(2E,4E)-2-HYDROXY-6-OXO-6-PHENYLHEXA-2,4-DIENOIC 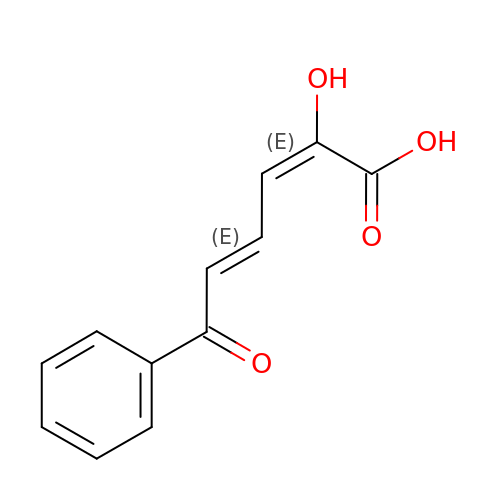ACID | C12 H10 O4 | RDRDHXDYMGUCKE-VCABWLAWSA-N>METKTETKTGTTNFDQEALLYHQQGKPGKIEVISSKPCATEKDLSLAYSPGVAAPCKAIAKDPAKVYDYTAKGNLVAVISNGTAVLGLGNIGPAAGKPVMEGKGILFKQFAGIDVFDIEVAATDVDTFCNAVRVLEPTFGGINLEDIKAPECFEIEERLKKEMNIPVFHDDQHGTAIVSGAALLNACSITNRKMEDMRIVVNGAGASANSCAKIFIALGARRENIIMCDSQGVIYKGRTAGMNKYKEYFASETEARTLTEALRGADVFVGLSVAGALTPEMLKDMAKDPIIFAMANPEPEITPDKARAARPDAIIATGRSDYPNQVNNVLGFPSIFRGALDTRSTQINEEMKLAAVHALAKLARMDVPDKVSATYGGKSFKFGRDYLIPKPFDTRVLLWVAPEVAKAAMKSGVATRAIEDWDQYRESLEAQQGPSKVFIRSAINRVHQNSEANGGELPRIVFPEGTSTKVLKALATLVEERICQPILLGYPERVKEKIKALDIPLLNDVQIVHPSSHPKYFSFVEKLYSLRQRKGINLGEAERLMADPNYFAAMMVNMGEADGMVSGSSINYADAVRPILQTIGTYKEGIPAGLNFVLLEDKFLVLADTTVNFNPSAEQCAQIALQAAKIVEYFGIEPRVAMLSYSNFSGAEGTPRKMKKAAEIARTLRPDLMIEGDMQADTAVNPEIMERLFPFSGLKGGANVLVFPNLESSNIAYKLIQQIGKAEVIGPFLTGVRRSANVLQRTTTVDGIVNSVVFTALEAQFIKDALKARGKK[6x]

While reducing NAD(P)+ to NAD(P)H, MEs catalyze the oxidative decarboxylation of the TCA cycle intermediate L-malate to produce the TCA carbon source pyruvate and a byproduct carbon dioxide (CO2) in the presence of divalent metal ions such as a magnesium (Mg2+) ion. The hybrid-type MEs consist of an N-terminal catalytic domain (ME domain) and a C-terminal activity regulating domain. The PTA domain does not possess an enzymatic activity of PTA but acts as an allosteric modulator of catalysis; that is, binding of some metabolites to the PTA domain increases or decreases the enzymatic activity. Binding of acetyl-CoA to the PTA domain is known to reduce the catalytic activity of several hybrid-type MEs.

Next, we collected data under the condition with acetyl-CoA (BbMaeBacetyl-CoA). In the result of 2D classification of the BbMaeBacetyl-CoA data, the ME domain of BbMaeBacetyl-CoA was relatively flexible as was observed in EcMaeB. We determined the structure of BbMaeBacetyl-CoA at 3.18 Å resolution. However, the obtained cryo-EM map of BbMaeBacetyl-CoA shows the C1 symmetry and not D3 because only one of 3 ME domain dimers clearly shows the V state. The states of the other 2 ME domain dimers are relatively ambiguous, implying incomplete transition from the H state. In the structure of BbMaeBacetyl-CoA, acetyl-CoA binds to two binding sites, binding sites 1 and 2. The binding site 1 is the same as where acetyl-CoA is found in the crystal structure of BbMaeB-HD. At the binding site 1, acetyl-CoA is stabilized through interactions with R531, K534, R577, and Q679. The binding site 2 is located near the linker helices, which connect the ME and PTA domains and hence are involved in the structural change from the H state to the V state. Acetyl-CoA at the biding site two is stabilized by hydrogen bonds with R737, R738, and R773, and by hydrophobic interaction with Y633.>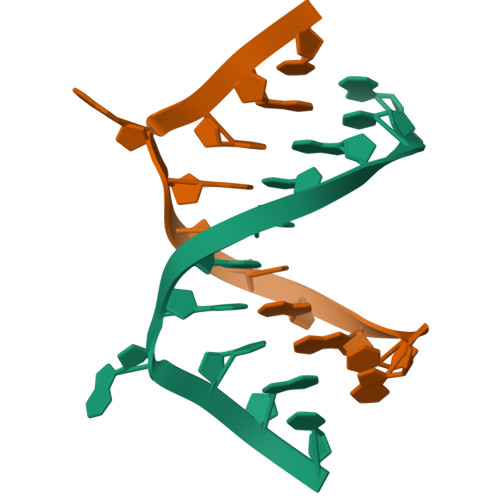GCGATATACGU[4x]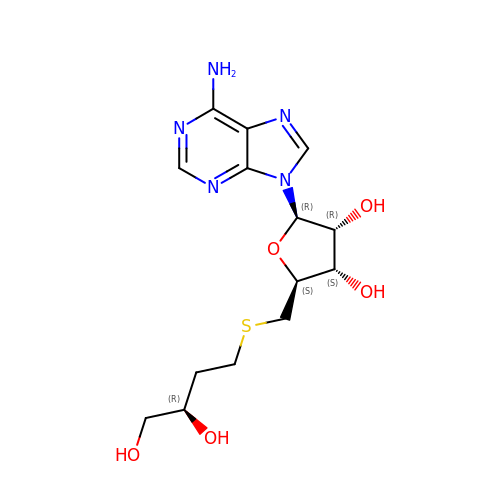5'-S-[(3R)-3,4-dihydroxybutyl]-5'-thioadenosine | C14 H21 N5 O5 S | QSBLNOGMFRGVGL-BAYCTPFLSA-N(2R)-2-azanyl-3-[(4-methoxyphenyl)-diphenyl-methyl]sulfanyl-propanoic 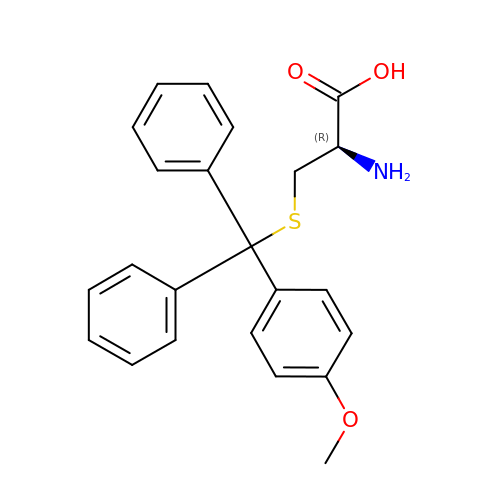acid | C23 H23 N O3 S | QAINHNNAIDVCEZ-NRFANRHFSA-N>[2x]MSTSLLFEQLNFLILVAAEAELPIAHSTRKLLMDNSCNNCQIYELYNENLKDVKTDKDWFMNKFGPQTVHFVISNTINFPFYKIVYFDLLIPVVSHTWVQDSVKTKRHLRTNMYSPNPFHLLRDCQVYISKSSFNKCEYILYSDLLHLLGGTLVNYISNRTTHVIVQSPQDPIIATVSKLTFGSFSSSSTNKHTEKPLREWKFVYPIWILYHFKMAKPLKGELATL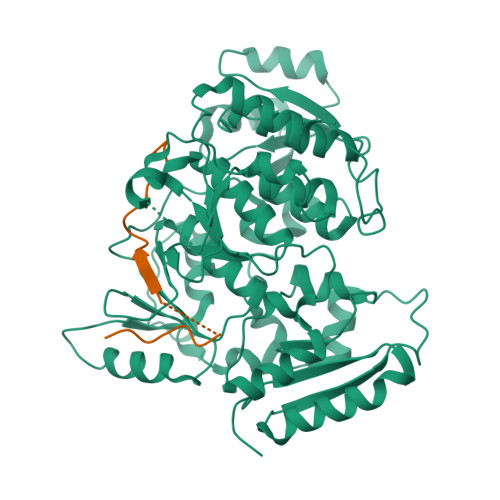CELDMQDTSEEQLFAKWEEVIGDKQTSSSQLTLHPNKTLFKNHHFAISPDLNFFTPLYWFLKGFIEDLDGKVTPLSFSDDLKSVYQAFPDIDCYIGHSANSPILEKTKSIKPEIHVGNVSWLFYMFALQKFTPVSQCKLIHQPFHAKLFTSKELTVAYTNYFGSQRFYIQRLVEILGGLSTPELTRKNTHLITKSTIGKKFKVAKKWSLDPQNAIIVTNHMWLEQCYMNNSKLNPKDSRFQNFKLDDNMGWNIGQIGMDHSSLPTPKNLSMVTYDTQSISEKPPPTN;>[2x]ETVPDSQISGFDSPLIPTSVGSYFRDDDD>[8x]KDWRDKDQSDGFGKVYVTEKVAQIKQIPFDASKLHSSPQMAAQHNMVDDGSGKVEIWRVENNGRIQVDQNSYGEFYGGDCYIILYTYPRGQIIYTWQGANATRDELTTSAFLTVQLDRSLGGQAVQIRVSQGKEPVHLLSLFKDKPLIIYKNGTSKKGGQAPAPPT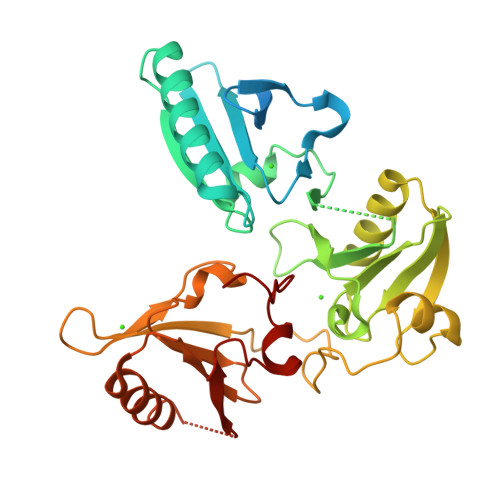RLFQVRRNLASITRIVEVDVDANSLNSNDVFVLKLPQNSGYIWVGKGASQEEEKGAEYVASVLKCKTLRIQEGEEPEEFWNSLGGKKDYQTSPLLETQAEDHPPRLYGCSNKTGRFVIEEIPGEFTQDDLAEDDVMLLDAWEQIFIWIGKDANEVEKKESLKSAKMYLETDPSGRDKRTPIVIIKQGHEPPTFTGWFLGWDSSKW> NMVHPNVICDGCNGPVVGTRYKCSVCPDYDLCSVCEG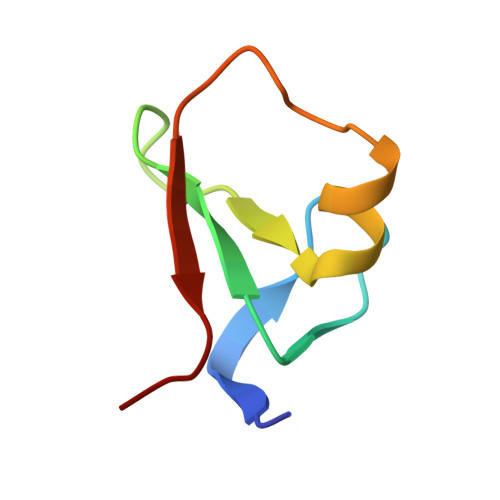KGLHRGHTKLAFPSPF> GAMGSYKDNIRHGVCWIYYPDGGSLVGEVNEDGEMTGEKIAYVYPDE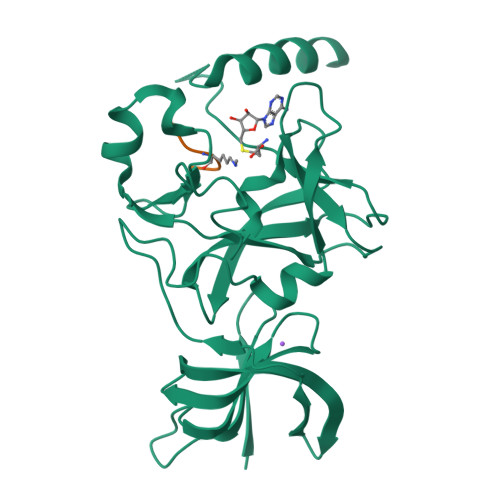RTALYGKFIDGEMIEGKLATLMSTEEGRPHFELMPGNSVYHFDKSTSSCISTNALLPDPYESERVYVAESLISSAGEGLFSKVAVGPNTVMSFYNGVRITHQEVDSRDWALNGATLSLDEETVIDVPEPYNHVSKYCASLGHKANHSFTPNCIYDMFVHPRFGPIKCIRTLRAVEADEELTVAYGYDHSPPGKSGPEAPEWYQVELKAFQATQQK;> SKSKDRKYTL>[4x]MRKKEDKYDFRALGLAIKEARKKQGLTREQVGAMIEIDPRYLT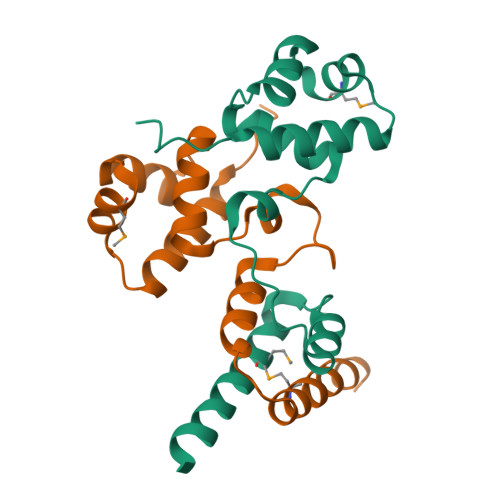NIENKGQHPSLQVLYDLVSLLNVSVDEFFLPASSQVKSTKRRQLENKIDNFTDADLVIMESVADGIVKSKEVGEMAGENLYFQ>[2x]MVPAAQQTATAPDAALTFPEGFLWGSATASYQIEGAAAEDGRTPSIWDTYARTPGRVRNGDTGDVATDHYHRWREDVALMAELGLGAYRFSLAWPRIQPTGRGPALQKGLDFYRRLADELLAKGIQPVATLYHWDLPQELENAGGWPERATAER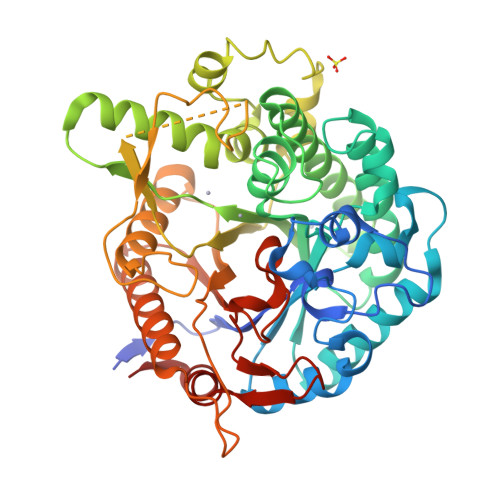FAEYAAIAADALGDRVKTWTTLNEPWCSAFLGYGSGVHAPGRTDPVAALRAAHHLNLGHGLAVQALRDRLPADAQCSVTLNIHHVRPLTDSDADADAVRRIDALANRVFTGPMLQGAYPEDLVKDTAGLTDWSFVRDGDLRLAHQKLDFLGVNYYSPTLVSEADGSGTHNSDGHGRSAHSPWPGADRVAFHQPPGETTAMGWAVDPSGLYELLRRLSSDFPALPLVITENGAAFHDYADPEGNVNDPERIAYVRDHLAAVHRAIKDGSDVRGYFLWSLLDNFEWAHGYSKRFGAVYVDYPTGTRIPKASARWYAEVARTGVLPTA> SGRGKGGKGLGAGG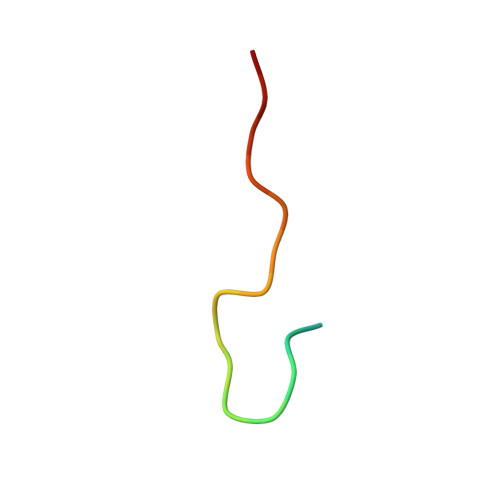AKRHRK PhoQ is the sensor kinase component of the PhoPQ two-component regulatory system that governs the phosphorylated state of the response regulator PhoP. PhoQ exists as a dimer within the inner membrane and has a periplasmic sensor domain (PD) that transduces signals across the inner membrane to the cytoplasmic histidine kinase domain. The PhoQ PD is a member of the PAS-fold and PDC-fold domain families. Unlike other PDC-sensors, which bind small ligands in a defined binding pocket or PhoQ PD homologs found in environmental bacteria, the PhoQ PD from bacteria that primarily interact with animals has no apparent binding pocket due to an occluding structural element: α-helices 4 and 5.

To test this hypothesis, we engineered a PhoQ PD mutant that contains an internal disulfide bond predicted to restrict conformational dynamics between α4 and α5 and the α/β-core. The PhoQW104C-A128C disulfide mutant was designed to inhibit motion between α2 and α4, allowing us to determine whether the dynamics of α4 and α5 play a critical role in activation. As predicted, the PhoQW104C-A128C PD formed an intramolecular disulfide bond between W104C and A128C, covalently linking α2 and α4 (inset). The protomers in the PhoQW104C-A128C PD structure are highly similar to each other, with an average root mean squared deviation (r.m.s.d.) of 0.3. The PhoQW104C-A128C PD is structurally similar to wild type and has increased stability. While the wild-type PhoQ PD unfolded with a Tmapp of 56°C in the presence and absence of TCEP, the PhoQW104C-A128C PD had a significantly increased Tmapp of 75°C. When reduced with TCEP, the PhoQW104C-A128C PD was slightly destabilized relative to the wild type, with a Tmapp 52°C. Therefore, the W104C-A128C disulfide increased the intrinsic stability of the PD at pH 5.5 relative to wild type. A disulfide bond between α-helices 2 and 4 inhibits PhoQ activation by acidic pH and divalent cation limitation, but does not inhibit activation by CAMP. Combined, these results suggest that the mechanism by which the W104C-A128C disulfide bond inhibits PhoQ activation by acidic pH and divalent cation limitation involves a loss of conformational flexibility between α4 and α5 and the α/β-core. In this study, we have shown that activation by acidic pH and divalent cation limitation are separable from CAMP-mediated activation by rigidifying the interaction between α4 and α5 and the α/β-core. The work in this study led to the construction of a specific S. enterica Typhimurium PhoQ mutant that is inhibited for activation by acidic pH or divalent cation limitation. This mutant has wild-type virulence in susceptible and resistant mouse models of systemic infection suggesting that, at least in these models, acidic pH and divalent cation sensing are dispensable for virulence.

>MDKTTFRLLRGESNLFYTLAKWENNKISVELPENLDMQSPTMTLIYDETGKLLWTQRNIPCLIKSIQPEWLKTNGFHEIETNVDCTSTLLSEDHSAQEKLKEVREDDDDAEMTHSVAVNIYPATARMPQLTIVVVDTIPIELKRSYMHHHHHH[3x]>MKKNLTNIYLIGLMGAGKTSVGSQLAKLTKRILYDSDKEIEKRTGADIA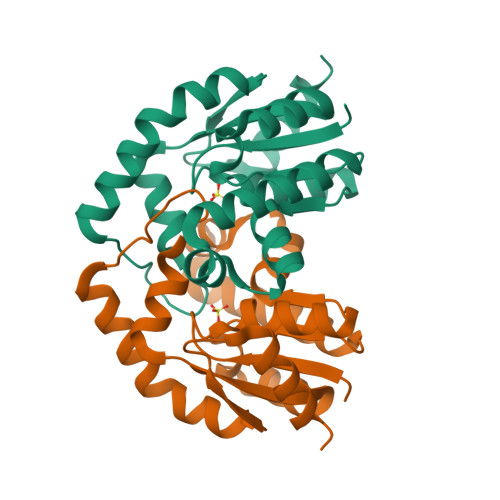WIFEMEGEAGFRRREREMIEALCKLDNIILATGGGVVLDEKNRQQISETGVVIYLTASIDTQLKRIGQKGEMRRPLFIKNNSKEKLQQLNEIRKPLYQAMADLVYPTDDLNPRQLATQILVDIKQTYSDLENLYFQ[2x]>EKEMIERDMREYRGFSRAVRAVFEEKERFPGLVDVVSNLIEVDEKYSLAVSVLLGGTAQNIVVRNVDTAKAIVEFLKQNEAGRVTILPLDLIDGSFNRISGLENERGFVGYAVDLVKFPSDLEVLGGFLFGNSVVVET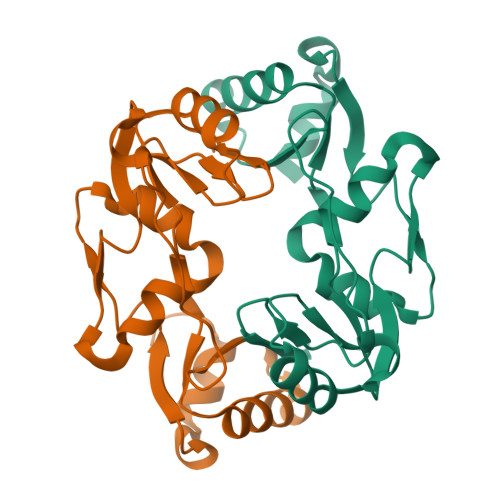LDDAIRMKKKYRLNTRIATLDGELISGRGAITGGREERSSNVFERRIK[4x]>MSVKQLGYLIFECRADVLEQMVVVYQDIIGAVVERDEGGRALVRLDGRPFRIRLDPGPANRLAAIGWNVDPSDLAAIAEQVEKACYSVVTADAELAADRAAAQVRQFADNDGFTHELYVESSFPTDPVLESLFVCGEEANGIFGLGHLVVIVADRAKTQSFFTDVLGFGLSDRVTWPEADIFFLHCNQRHHTVALSAPALGLKPGMVHHLMLEAKSKEQVDRAFAAVKRLGYDVLMTIGQHSNDKVYSFYMMAPAGFAVELGFGGQVIGDLESWHVGFYDAPSIWGHELQLPAH[4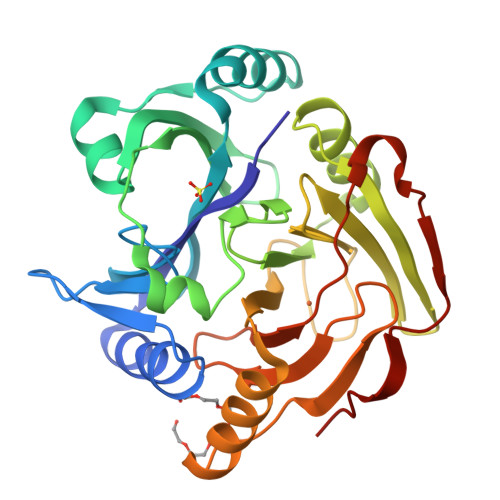x]>[3x]MHHHHHHHHSSGLVPRGSAM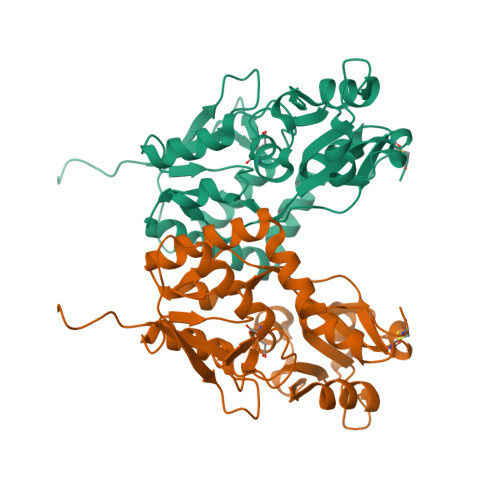GSKPLRIGVPNRVSYTDYVSKDKNPPGVRGYCIDVFEAAIELLPYPVPRTYILYGDGKRNPSYDNLVNEVVADNFDVAVGDITIVTNRTRYVDFTQPFIESGLVVVAPVKEAGTIEGIDSLVTSNEPIGVQDGTFARNYLINELNILPSRIVPLKDEEQYLSALQRGPNAGGVAAIVDELPYIEVLLTNSNCKFRTVGQEFTRTGWGFAFQRDSPLAVDMSTAILQLSEEGELEKIHRKWLNYKHECS>MHSLMKPTREPQINLFKKSNPYKAKVISNVLLTPETGTGKRPKKEGEALVHRIVLAIDHSAYPYVIGQSGGVIPPGEDPEKKAKGLADVGYTVRLYSIASPSYSFGMKEDNIEFIIKRDNIYDENGNIQFKGVCSNYMCDLKPGDEVTMTGPSGKKFLLPNTDFSGDIMFLATGTGIAPFIGMSEELLEHKLIKFTGNITLVYGAPYSDELVMMDYLKGLESKHKNFKLITAISREEKNSFDGGRMYISHRVREQAEAVKKILNGGGRFYICGGPKGMEKGVIEEIQKISGNTGTYEEFKHHLEGAH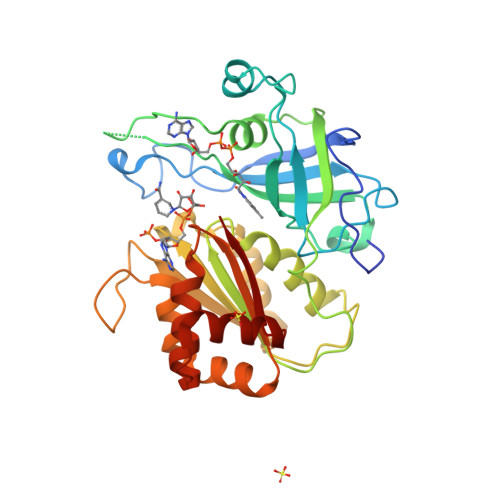QLFVETY[4x]> MKNIGWMLRQRATVSPRLQAYVEPSTDVRMTYAQMNALANRCADVLTALGIAKGDRVALLMPNSVEFCCLFYGAAKLGAVAVPINTRLAAPEVSFILSDSGSKVVIYGAPSAPVIDAIRAQADPPGTVTDWIGADSLAERLRSAAADEPAVECGGDDNL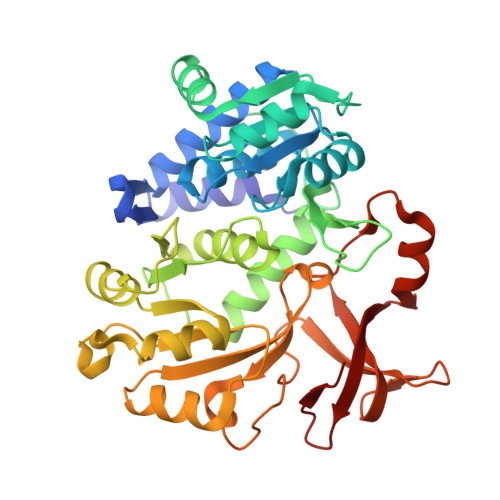FIMYTSGTTGHPKGVVHTHESVHSAASSWASTIDVRYRDRLLLPLPMFHVAALTTVIFSAMRGVTLISMPQFDATKVWSLIVEERVCIGGAVPAILNFMRQVPEFAELDAPDFRYFITGGAPMPEALIKIYAAKNIEVVQGYALTESCGGGTLLLSEDALRKAGSAGRATMFTDVAVRGDDGVIREHGEGEVVIKSDILLKEYWNRPEATRDAFDNGWFRTGDIGEIDDEGYLYIKD>EIQEAYILSGARTPTAKFNGSFVSVSAPELGAVAIKSAVSKSGVPVEKITDVYMGNVLQGAVGQAPARQASMFAGLSPTVESMTVNKVCASGLKAVALAAQNIQLGLAEAQVAGGMENMSRVPYYLPRSTQLPPFGEIKLQDGLIQDGLWDVYNQFHMGICAEKTAKKYEISREEQDQYAIQSYQRAQAAWKENKFAEEIAPVTVKGKKGETVVERDEGYENLRIDKMATLKPAFLRDGTGTVTAGNASTMNDGASALVLGSKAIAREFAQGNRALARIVSTADAAIDPVDFPVAPAKAVPIALERAGITKDQVAVWEFNEAFAAVIKANEKILGLQNARVNPLGGAISLGHALGSSGSRILVTLLHQLQPGEYGVAAICNGGGAATAMVVQKLDRV[4x]

In this study, we have characterized recombinant AfERG10A as a functional acetyl-CoA acetyltransferase catalyzing both synthetic and degradative reactions. Unexpectedly, AfERG10A localizes to the mitochondria in A. fumigatus, as shown by C-terminal green fluorescent protein (GFP) tag fusion. Both knockout and inducible promoter strategies demonstrate that Aferg10A is essential for the survival of A. fumigatus. AfERG10A consists of three domains, an N-terminal domain (residues Glu36 to Asn153 and Asn287 to Arg302), a C-terminal domain (residues Ala312 to Asp433), and a loop domain (residues Met154 to Met286).

To provide insight into the structural prerequisites and find potential exploitable differences between AfERG10A and human orthologues, structures of apo- and CoA-complexed AfERG10A were determined using crystals grown from conditions of 0.1 M HEPES (pH 7.0) and 2 M ammonium sulfate in the absence or presence of CoA. In one asymmetric unit, there are four molecules (A to D) forming a tetramer, which is similar to other members of thiolase family, such as in humans, S. cerevisiae, and E. coli. The N-terminal and C-terminal halves have a βαβαβαββ topology and are connected by the loop domain of approximately 130 residues. By comparison, the root mean square deviation (RMSD) value between the apo- and CoA-bound structures is 0.175 Å, with 367 atoms matched, suggesting that CoA binding does not cause major conformation change. Sequence alignment of AfERG10A with ACAT1 and ACAT2 revealed that the equivalent catalytic residues are Cys124, His387, and Cys415 in AfERG10A. To confirm this, point mutations were introduced at the three sites as C124S, H387F, and C415S, and activity assays were conducted. As expected, the activity of these mutation variants could not be detected in either direction (data not shown), suggesting that these residues are essential for the catalytic activity of AfERG10A.(4~{S})-5-[4-[[4-(2-ethyl-2-oxidanyl-butoxy)-3-methyl-phenyl]-dimethyl-silyl]-2-methyl-phenoxy]-4-oxidanyl-pentanoic 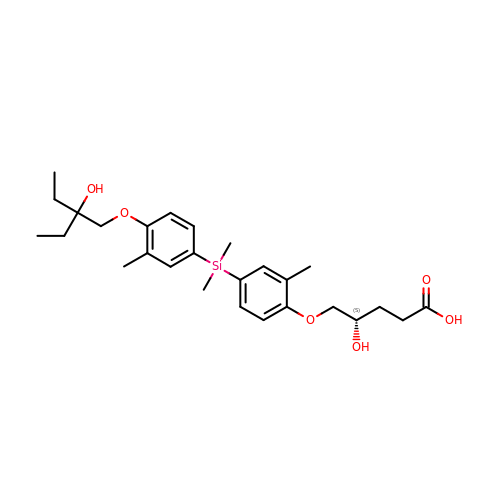acid | C27 H40 O6 Si | ZRDFZSBOZQJKGC-NRFANRHFSA-N>[4x]MDTNKREIVEFLGIRTYFFPNLALYAVNNDEL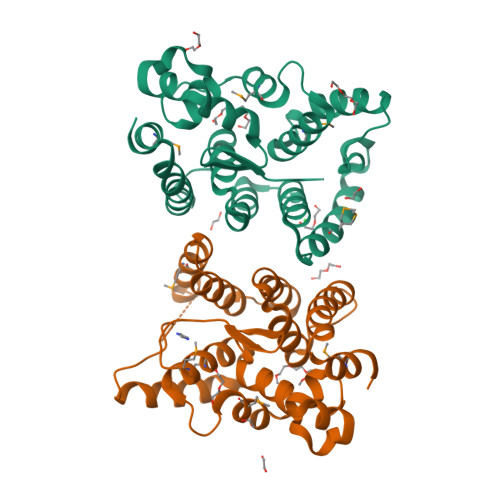LVSDPNKANSFAAYVFGASDKKPSVDDIVQMLFPSGSDSGTILTSMDTLLALGPDFLTEFKKRNQDLARFNLTHDLSILAQGDEDAAKKKLNLMGRKAKLQKTEAAKILAILIKTINSEENYEKFTELSELCGLDLDFDAYVFTKILGLEDEDTADEVEVIRDNFLNRLDQTKPKLADIMRNGP>[4x]MRTSKKEMILRTAIDYIGEYSLETLSYDSLAEATGLSKSGLIYHFPSRHALLLGMHELLADDWDKELRDITRDPEDPLERLRAVVVTLAENVSRPELLLLIDAPSHP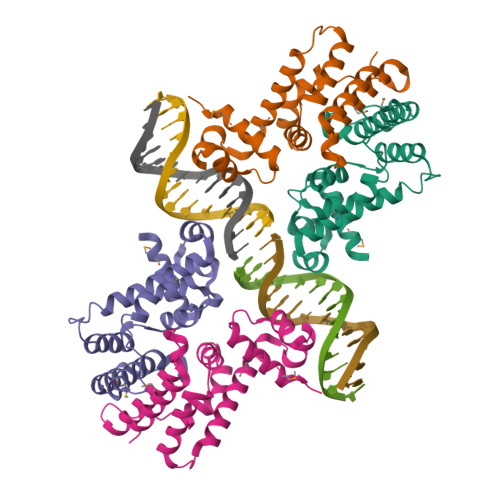DFLNAWRTVNHQWIPDTDDLENDAHKRAVYLVQLAADGLFVHDYIHDDVLSKSKRQAMLETILELIPSQT>LYFQSMMLDRIRVVLVNTSHPGNIGGAARAMKNMGLSQLVLVQPESFP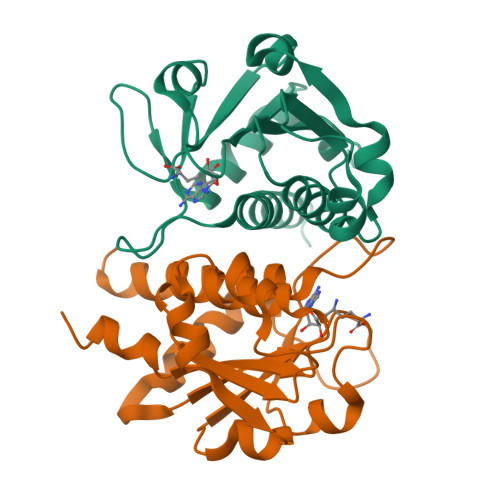HGDAVARASGATDILDAARVVDTLEEALSGCSVVLGTSARDRRIPWPLLDPRECATTCLEHLEANGEVALVFGREYAGLTNEELQRCQFHVHIPSDPEFGSLNLAAAVQVLTYEVRMAWLAAQGK[4x]> MAIGDIQTSVAFDRQVGRFPPR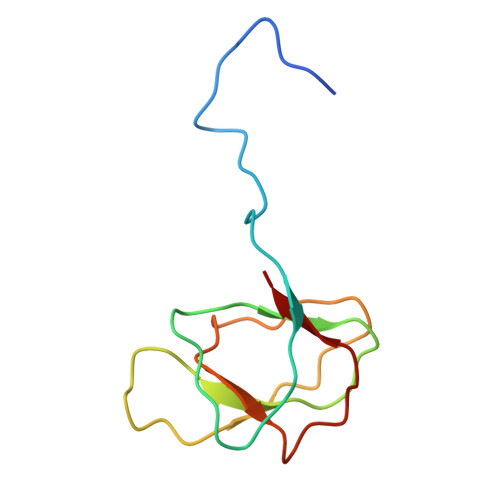AEVVTPSNSEEFTSGVSVFSNDGGDISVVPLLPYGSAAIVVTVAAGGFVPFMVRKVNATGTTSTSIVAVW> MRCLAAGVHYKTLIVICALLSLLTVLLWNKCTSEKALRFLPQHPQPPPSPKIDSHPQQPQPPEPPPVVGGVRYEEIDCLINDDATIKGRREGSEVYMPFSWMEKYFEVYGKVVQYDGYDRFEFSHSYSKVYAQREQYHPNGVFMSFEGYNVEVRDRVKCISGVEGVPLSTQWGPQGYFYAIQIAQYGLSHYSKNLTER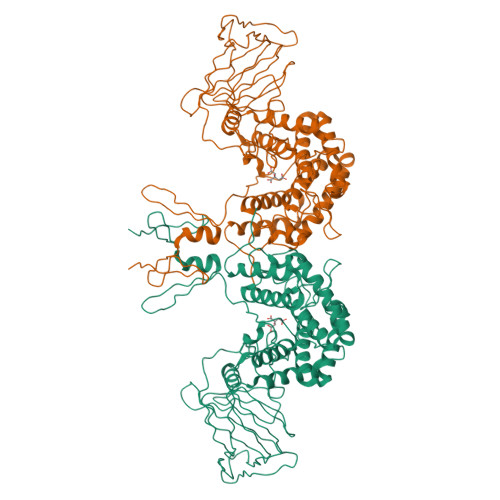PPHVEVYDTAEERDSRSSAWTVPKGCSLTRVYDKTRATSVREFSAPENSEGVSLPLGNTKDFIISFDLKFTSNGSVSVILETTEKGPPFVIHYVTTTQLILLKDRDITYGIGPRTTWTTVTRDLLTDLRKGIGLSNTKAVKATKTMPRRVVKLVVHGTGTIDNITISTTSHMAAFYAASDWLVRNQDERGGWPIMVTRKLGEGFRALEPGWYSAMAQGQAMSTLVRAYLMTKDDRYLKAALRATGPFKLPSEQHGVKAVFMNKYDWYEEYPTIPSSFVLNGFIYSLIGLFDLAQTAGEKLGRDAGQLYSKGMESLKVMLPLYDTGSGTIYDLRHFILGTAPNLARWDYHTTHINQLQLLGTIDNSPIFRDSVKRWKSYLKGGRAKHN>[2x]MAKKTSSVPRTVLPFEAMPRRPGNRWLRLLQIWREQGYEDLHLEVHQTF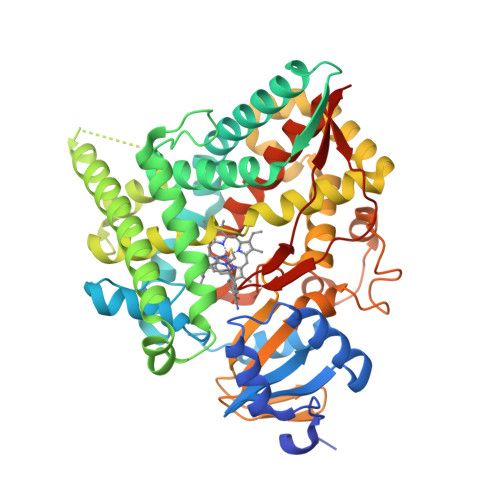QELGPIFRYDLGGAGMVCVMLPEDVEKLQQVDSLHPHRMSLEPWVAYRQHRGHKCGVFLLNGPEWRFNRLRLNPEVLSPNAVQRFLPMVDAVARDFSQALKKKVLQNARGSLTLDVQPSIFHYTIEASNLALFGERLGLVGHSPSSASLNFLHALEVMFKSTVQLMFMPRSLSRWTSPKVWKEHFEAWDCIFQYGDNCIQKIYQELAFSRPQQYTSIVAELLLNAELSPDAIKANSMELTAGSVDTTVFPLLMTLFELARNPNVQQALRQESLAAAASISEHPQKATTELPLLRAALKETLRLYPVGLFLERVASSDLVLQNYHIPAGTLVRVFLYSLGRNPALFPRPERYNPQRWLDIRGSGRNFYHVPFGFGMRQCLGRRLAEAEMLLLLHHVLKHLQVETLTQEDIKMVYSFILRPSMFPLLTFRAINHHHH Glycinamide-RNase-transformylase T (PurT) is found only in some specific bacteria including Mtb and utilizes ATP-dependent ligation to catalyze the formylation of 5′-phosphoribosyl-glycinamide (GAR) in the third reaction of the de novo purine salvage pathway. Structural comparisons of MtbPurT using DALI Server indicated that it was structurally similar to the ATP-grasp fold proteins with their characteristic three domains, and thus MtbPurT is categorized as a member of the ATP-grasp superfamily as in the previous studies. According to the MtbPurT structure, the monomer of MtbPurT consists of a small lid domain and a large α/β domain. The B-domain forms a flexible lid and covers the active site for ATP binding.

The MtbPurT crystal diffracted at 2.79 Å resolution at the SSRF and belonged to a space group P3121. There were two MtbPurT molecules in the asymmetric unit. Therefore, the MtbPurT protein exists as a dimer in solution. The final structure of MtbPurT is well ordered, and electron densities for all residues were clearly interpretable, except in four parts (residues 111–113, 175–180, 189–198 and 205–215). In contrast to phBCCPPurT, loop 252–255 between β11 and β12 in MtbPurT shifted by 13.1 Å away from the cofactor binding site. This structural rearrangement in apo-MtbPurT represents an “open” conformation. As a result, the pocket of MtbPurT for the cofactor binding has a much broader opening with a width of 11.6 Å (distance between Ser182 and Asp251) than 7.3 Å (distance between Ser172 and Asp239) for phBCCPPurT. And MtbPurT recognizes ATPγS with a relatively low binding affinity, with the Kd value of 207.41 ± 8.02 μM. All four mutants (R131A, E217A, S218A and V220A) lost their ATP-binding capability, indicating essential roles for these residues in binding with ATP. In particular, loop 383–389 in MtbPurT is much shorter than that in EcPurT (loop 352–364) and shifted 5.7 Å away from the phosphate of the GAR substrate; thus, no hydrogen bonds with GAR were found.

>[2x]MVIDGWTEEQHEPTVRHERPAAPQDVRRVMLLGSAEPSRELAIALQGLGAEVIAVDGYVGAPAHRIADQSVVVTMTDAEELTAVIRRLQPDFLVTVTAAVSVDALDAVEQADGECTELVPNARAVRCTADREGLRRLAADQLGLPTAPFWFVGSLGELQAVAVHAGFPLLVSPVAGVAGQGSSVVAGPNEVEPAWQRAAGHQVQPQTGGVSPRVCAESVVEIEFLVTMIVVCSQGPNGPLIEFCAPIGHRDADAGELESWQPQKLSTAALDAAKSIAARIVKALGGRGVFGVELMINGDEVYFADVTVCPAGSAWVTVRSQRLSVFELQARAILGLAVDTLMISPGAARVINPDHTAGRAAVGAAPPADALTGALGVPESDVVIFGRGLGVALATAPEVAIARERAREVASRLNVPDSRE>GSSLPKPILRVQPDSVVSRWTKVTFFCEETIGANEYRLYKDGKLYKTVTKNKQKPANKAEFSLSNVDLSNAGQYECSYSTQYKSSGYSDPLKLVVTGHYWTPSLLAQASPVVTSGGYVTLQCESWHNDHKFILTVEGPQKLSWTQDSQYNYSTRKYHALFSVGPVTPNQRWICRCYSYDRNRPYVWSPPSESVELLVSGNLQKPTIKAEPGSVITSKRAMTIWCQGNLDAEVYFLHNEGSQKTQSTQTLQQPGNKGKFFIPSMTRQHAGQYRCYCYGSAGWSQPSDTLELVVTGIYEHYKPRLSVLPSPVVTAGGNMTLHCASDFHYDKFILTKEDKKFGNSLDTEHISSSRQYRALFIIGPTTPTHTGTFRCYGYFKNAPQLWSVPSDLQQILISGLSKKPSLLTHQGHILDPGMTLTLQCYSDINYDRFALHKVGGADIMQHSSQQTDTGFSVANFTLGYVSSSTGGQYRCYGAHNLSSEWSASSEPLDILITGQLPLTPSLSVKPNHTVHSGETVSLLCWSMDSVDTFILSKEGSAQQPLRLKSKSHDQQSQAEF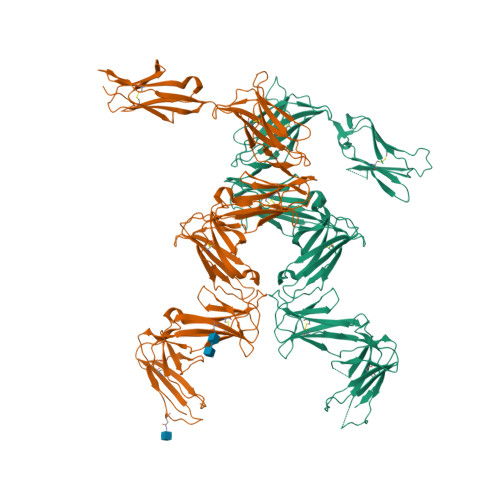SMSAVTSHLSGTYRCYGAQNSSFYLLSSASAPVELTVSGAAAHHHHHH[2x]> MSEPMMWLLVRGVWETLAMTFVSGFFGFVIGLPVGVLLYVTRPGQIIAN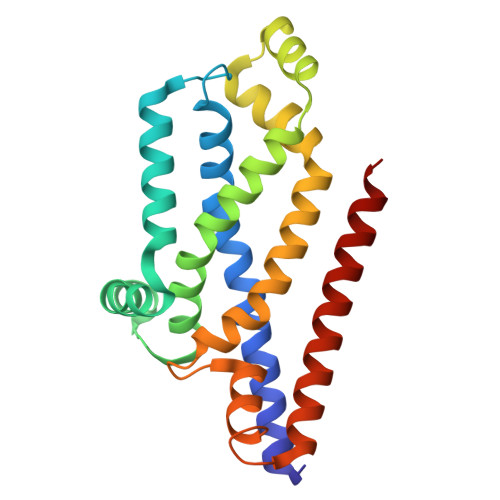AKLYRTVSAIVNIFRSIPFIILLVWMIPFTRVIVGTSIGLQAAIVPLTVGAAPFIARMVENALLEIPTGLIEASRAMGATPMQIVRKVLLPEALPGLVNAATITLITLVGYSAMGGAVGAGGLGQIGYQYGYIGYNATVMNTVLVLLVILVYLIQFAGDRIVRAVT(3R)-1-[(4R)-AZEPAN-4-YLCARBAMOYL]-3-(SULFOAMINO)-L-PROLINE 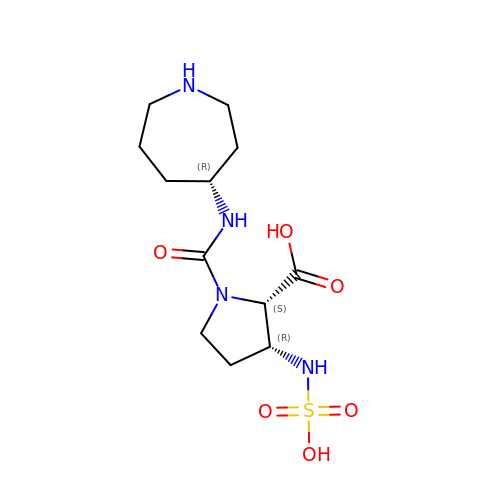| C12 H22 N4 O6 S | WWLDRJMXWRULQB-BBBLOLIVSA-N To advance the understanding of esterases, we have identified and characterized E53, an alkalophilic esterase from a marine bacterium Erythrobacter longus. Family IV esterases, to which E53 belongs, are widely distributed in microorganisms, plants, and animals, specifically degrade short-chain esters. The family IV esterase can be characterized by the α/β-fold hydrolase group, and contains two distinct structural domains: an N-terminal CAP domain and a C-terminal catalytic domain. The catalytic reaction relies on the S-H-D/E catalytic triad located in the catalytic domain.

The catalytic triad was composed of S162, D254, and H284. We have prepared S162A, D254A and H284A variants and mutating the three residues to alanine (S162A, D254A, H284A) resulted in almost total loss of activity. The serine initiates the reaction by attacking carbonyl carbon of esters, while histidine and aspartic acid/glutamic acid facilitate the proton transfer from the serine to histidine residue. The distances among the catalytic triad in WT and mutated E53 were 2.6–2.9 Å for H284Nε2 to S162Oγ and 2.5–2.6Å for H284Nδ1 to D254Oδ2.

>[4x]MTDTPFIRPDMKAFLEAIAAMAGPTLAEMTLEEARASYVALHGMADRPARELAVIRNLSCPGPAGDIPLRLYDARESREAGPVITFYHGGGFVIGDLDTHHNLCTEIAALMDLPVVAVDYRLAPEHPFPAAIEDCEAATRWVASSPSELGRTASGVIPIGDAAGGNATIVVSQLLGAKPADVPVVLQVPIFPLASDAVGSASLEAFAEGFVLTKASIEFFDTAYKADRADPRGFPILGDHTAAPPTIVATASLDPIRDSGRDYAKALVEAGRDVVYLEMEGVTHSFTNIRAAVPSTQGDLERIIAAMKMMLGTA SHMT is a pyridoxal-5′-phosphate (PLP)-dependent enzyme that catalyzes the interconversion of l-serine (l-Ser) and tetrahydro­folate (THF) to glycine (Gly) and methylene tetrahydrofolate (MTHF). The enzyme provides activated one-carbon units for the synthesis of dTMP, choline and amino acids. Plasmodium serine hydroxymethyltransferase (SHMT) has recently been shown to be vital for parasite growth and development, making it a potential target for antimalarial drug development. The overall structure of PvSHMT was found to be very similar to that of PfSHMT, existing as a twofold symmetric homodimer with two catalytic sites.

Furthermore, as in P. falciparum SHMT, a redox switch created from a cysteine pair (Cys125–Cys364) was observed. A previous study revealed that the THF-dependent activity of PfSHMT is regulated by the redox status of a cysteine pair. Sequence conservation (Cys125 and Cys364) and the presence of the sulfhydryl form in the PvSHMT–d-Ser–5FTHF and PvSHMT–l-Ser complexes and the disulfide in the PvSHMT–PLP structure prompted an examination of the dependence of PvSHMT activity on its redox state. Switching of enzyme activity based on the redox environment was also observed for PvSHMT.

>[3x]MFNNEPLEQIDKELHDILADEEKRQRETINLIASENLTNGAVRECLGNRVSNKYSEGYPKKRYYGGNDFIDKIEELCQKRALEAFNVSDEEWGVNVQPLSGSAANVQALYALVGVKGKIMGMHLCSGGHLTHGFFDEKKKVSITSDMFESKLYKCNSQGYVDLDAVREMALSFKPKVIICGYTSYPRDIDYQQFRQICDEVNAYLFADISHISSFVACNILNNPFLHADVVTTTTHKILRGPRSALIFFNKKRNPGIEQKINSAVFPSFQGGPHNNKIAAVACQLKEVHSPAFKEYTQQVLLNSKALAKALISKQIDLVTNGTDNHLIVVDLRKFSITGSKLQETCNAINVSLNKNTIPSDVDCVSPSGVRIGTPAMTTRGAKEKDMEFIADVLARAIKITVDLQEQYGKKLVDFKKGLPGNAQLQQLKQEVVTWAGALPFP>[6x]SNAMSTIARRGFHYMQRLNSANVSPALLEKAQNRVIDAALTFIRERAKFKGELMRSLGGVAATSSLLGVPLGHHSSFHEGSAF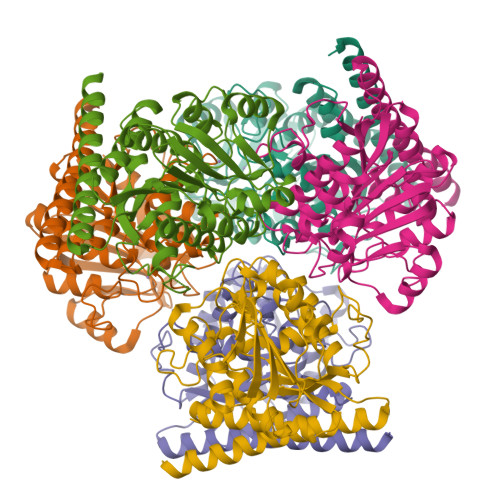APPRIREAIWCDSTNSTTEEGKNLRDPRVITNVGDVPIEEIRDCGVDDKRLANVISESVKLVMDEDPLRPLVLGGDHSISFPVVRAVSEKLGGAVDILHFDAHPDLYHDFEGNYYSHASPFARIMEGGYARRLVQVGIRSITNDVREQVKKYGVETHEMRTLSRDRPILENLKLGEGVKGVYVSIDVDSLDPSIAPGVSHHEPGGLLFRDILNILQNLQGDIVGGDVVEYNPQRDTYDGITALVAAKLVRELAAKMSK> MPVCKNCHGTEFERDLSNANNDLVCKACGVVSEDNPIVSEVTFGETSAGAAVVQGSFIGAGQSHAAFGGSSALESREATLNNARRKLRAVSYALHIPEYITDAAFQWYKLALANNFVQGRRSQNVIASCLYVACRKEKTHHMLIDFSSRLQVSVYSIGATFLKMVKKLHITELPLADPSLFIQHFAEKLDLADKKIKVVKDAVKL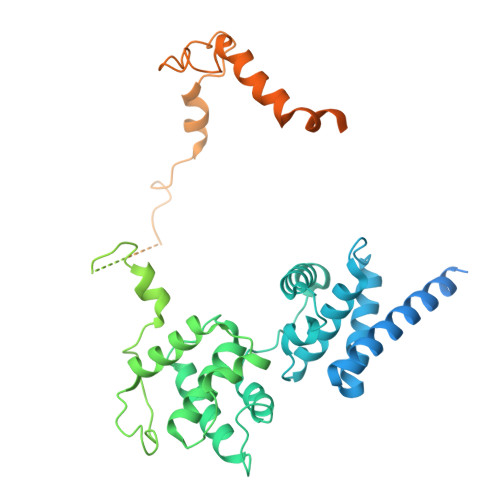AQRMSKDWMFEGRRPAGIAGACILLACRMNNLRRTHTEIVAVSHVAEETLQQRLNEFKNTKAAKLSVQKFRENDVEDGEARPPSFVKNRKKERKIKDSLDKEEMFQTSEEALNKNPILTQVLGEQELSSKEVLFYLKQFSERRARVVERIKATNGIDGENIYHEGSENETRKRKLSEVSIQNEHVEGEDKETEGTEEKVKKVKTKTSEEKKENESGHFQDAIDGYSLETDPYCPRNLHLLPTTDTYLSKVSDDPDNLEDVDDEELNAHLLNEEASKLKERIWIGLNADFLLEQESKRLKQEADIATGNTSVKKKRTRRRNNTRSDEPTKTVDAAAAIGLMSDLQDKSGLHAALKAAEESGDFTTADSVKNMLQKASFSKKINYDAIDGLFR4-[(2-methylsulfonylimidazol-1-yl)methyl]-1,3-thiazole | C8 H9 N3 O2 S2 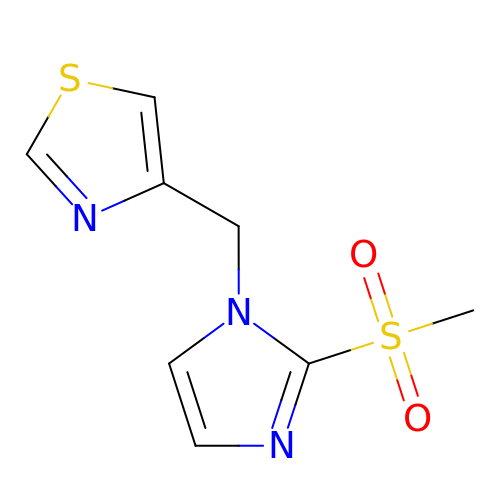| DWPGGNJRLYKHCD-UHFFFAOYSA-N>MKTLLKNSLTFLLMLMPVLAFAQQAPQ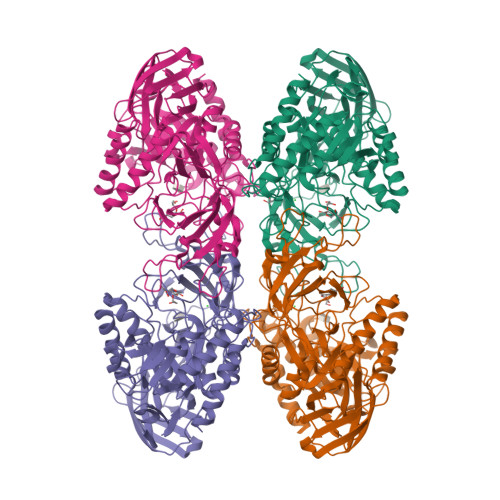IMNVSARQTTSLDGQWKTIVDPFENGYYDYRLKPYDGGYAQDKTYSDKTKLQEYDFETDKLLFVPGDWNTQRPQLYYYEGTVWYRKHFEYSLQPGKRLFLNFGAVNYEAIVWLNGKRLGRHIGGFTPFNFEITNLLKEGTNSLVVKVDNKRLPEAVPTVNADWWNFGGITRPVTLIEMPATYIRDYYVQLAKDDKNMIEGWVQLEGSDKEQKITLDIPELKVKKEVTTDANGYASFLIKSKPILWTPENPKLYAVNLASETDKVSDEIGFRTIRTEGIKILLNDKEIFCRGISIHEETPYYSGRAYSKDHAHTLLSWAKELGCNFVRLAHYPHNEEMVREAERMGFLVWSEIPVYWTIHWENKDTYQNAEQQLCDMIARDKNRCNIIIWSIANETPHSKTRLTFLSNLANKARSLDSVRLIGAAMEKEEVQPGVLTVNDPLGELLDIISFNEYVGWYDGDSEKCDRVNWTFDTQKPVFISELGGGALYGHHGSPKERFTEEYQEDLYIRHVNMLKRIPGLAGTTPWILKDFRSPRRHVPEIQDDFNRKGLVSDKGQKKKAFFVLQKWYKELTEAYK[6x]>[3x]MYSVLKQSIRPRLLATHNQFRTMITAQAVLYTQHGEPKDVLFTQSFEIDDDNLAPNEVIVKTLGSPINPSDINQIQGVYPSKPAKTTGFGTAEPAAPCGNEGLFEVIKVGSNVSSLEAGDWVIPSHVNFGTWRTHALGN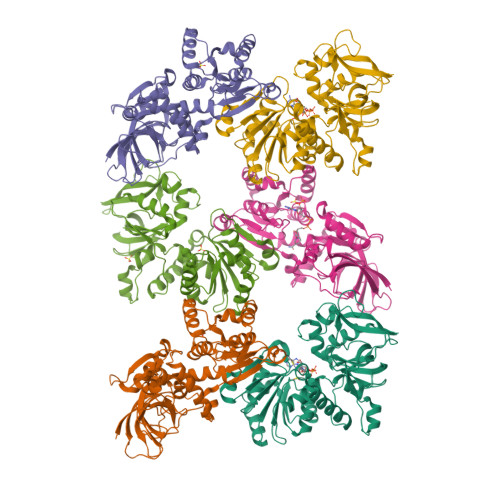DDDFIKLPNPAQSKANGKPNGLTINQGATISVNPLTAYLMLTHYVKLTPGKDWFIQNGGTSAVGKYASQIGKLLNFNSISVIRDRPNLDEVVASLKELGATQVITEDQNNSKEFGPTIKEWIKQSGGEAKLALNCVGGKSSTGIARKLNNNGLMLTYGGMSFQPVTIPTSLYIFKNFTSAGFWVTELLKNNKELKTSTLNQIIAWYEEGKLTDAKSIETLYDGTKPLHELYQDGVANSKDGKQLITY;>[3x]MYSVLKQSIRPRLLATHNQFRTMITAQAVLYTQHGEPKDVLFTQSFEIDDDNLAPNEVIVKTLGSPVNPSDINQIQGVYPSKPAKTTGFGTTEPAAPCGNEGLFEVIKVGSNVSSLEAGDWVIPSHVNFGTWRTHALGNDDDFIKLPNPAQSKANGKPNGLTINQGATISVNPLTAYLMLTHYVKLTPGKDWFIQNGGTSAVGKYASQIGKLLNFNSISVIRDRPNLDEVVASLKELGATQVITEDQNNSREFGPTIKEWIKQSGGEAKLALNCVGGKSSTGIARKLNNNGLMLTYGGMSFQPVTIPTSLYIFKNFTSAGFWVTELLKNNKELKTSTLNQIIAWYEEGKLTDAKSIETLYDGTKPLHELYQDGVANSKDGKQLITY TMEM16K is a widely distributed, but relatively unstudied member of the TMEM16 family. Here we show that TMEM16K is an ER-resident lipid scramblase with non-specific ion channel activity and a dependence on calcium ions and short chain lipids for optimum activity. We present structures of TMEM16K solved by both X-ray crystallography and cryo-electron microscopy, revealing a classic scramblase fold, with extensive conformational changes propagated from the cytoplasmic to the ER face of the membrane, which lead to opening or closing of the lipid transporting groove. The TM domain of TMEM16K is C-terminal to the cytoplasmic domain and has ten TM α helices with TM3 to TM7 forming the lipid scramblase ‘groove’ and TM6 to TM8 forming the binding site for two Ca2+ ions, seen in other TMEM16s.

To understand the structural basis of lipid scrambling in TMEM16K, we initially solved its structure by X-ray crystallography. We obtained preliminary diffraction data from vapour diffusion (VD) crystals of full-length human TMEM16K, which we improved by lipidic cubic phase (LCP) crystallisation to obtain 3.4 Å resolution data. Both structures were solved by molecular replacement (Methods section). The structures were similar (monomer all atom root mean square deviation (r.m.s.d.) = 0.75 Å), although the crystal packing differs, confirming that the conformation is not dictated by crystal contacts. All the protein samples used in cryo-EM were purified in the detergent undecyl maltoside (UDM) with cholesteryl hemisuccinate (CHS) added to improve protein stability: the same lipid detergent combination that was used for the VD crystallisation. A fourth Ca2+ ion site on the ER side of the membrane at the dimer interface was seen only in the LCP crystallisation, not in the VD or other structures, so this site is likely to be the result of the crystallisation conditions, not a characteristic of the protein or this conformation.

>[2x]MKVTLSALDTSESSFTPLVVIELAQDVKEETKEWLKNRIIAKKKDGGAQLLFRPLLNKYEQETLENQNLYLVGASKIRMLLGAEAVGLVKECNDNTMRAFTYRTRQNFKGFDDNNDDFLTMAECQFIIKHELENLRAKDEKMIPGYPQAKLYPGKSLLRRLLTSGIVIQVFPLHDSEALKKLEDTWYTRFALKYQPIDSIRGYFGETIALYFGFLEYFTFALIPMAVIGLPYYLFVWEDYDKYVIFASFNLIWSTVILELWKRGCANMTYRWGTLLMKRKFEEPRPGFHGVLGINSITGKEEPLYPSYKRQLRIYLVSLPFVCLCLYFSLYVMMIYFDMEVWALGLHENSGSEWTSVLLYVPSIIYAIVIEIMNRLYRYAAEFLTSWENHRLESAYQNHLILKVLVFNFLNCFASLFYIAFVLKDMKLLRQSLATLLITSQILNQIMESFLPYWLQRKHGVRVKRKVQALKADIDATLYEQVILEKEMGTYLGTFDDYLELFLQFGYVSLFSCVYPLAAAFAVLNNFTEVNSDALKMCRVFKRPFSEPSANIGVWQLAFETMSVISVVTNCALIGMSPQVNAVFPESKADLILIVVAVEHALLALKFILAFAIPDKPRHIQMKLARLEFESLEALKQQQMKLVTENLKEEPMESGKEKATAENLYFQ> MTISEARLSPQVNLLPIKRHSNEEVEETAAILKKRTIDNEKCKDSDPGFGSLQRRLLQQLYGTLPTDEKIIFTYLQDCQQEIDRIIKQSIIQKESHSVILVGPRQSYKTYLLDYELSLLQQSYKEQFITIRLNGFIHSEQTAINGIATQLEQQLQKIHGSEEKIDDTSLETISSGSLTEVFEKILLLLDSTTKTRNEDSGEVDRESITKITVVFIFDEIDTFAGPVRQTLLYNLFDMVEHSRVPVCIFGCTTKLNILEYLEKRVKSRFSQRVIYMPQIQNLDDMVDAVRNLLTVRSEISPWVSQWNETLEKELSDPRSNLNRHIRMNFETFRSLPTLKNSIIPLVATSKNFGSLCTAIKSCSFLDIYNKNQLSNNLTGRLQSLSDLELAILISAARVALRAKDGSFNFNLAYAEYEKMIKAINSRIPTVAP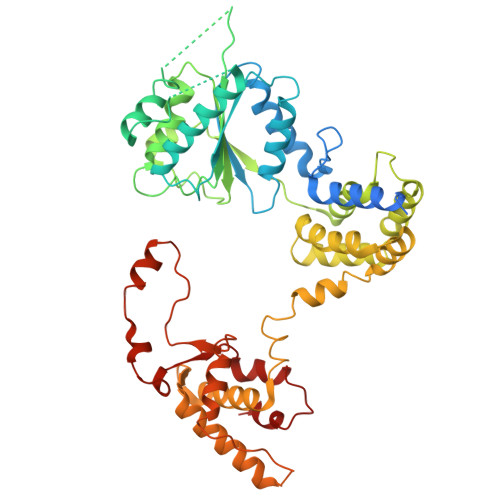TTNVGTGQSTFSIDNTIKLWLKKDVKNVWENLVQLDFFTEKSAVGLRDNATAAFYASNYQFQGTMIPFDLRSYQMQIILQELRRIIPKSNMYYSWTQL(6S)-2-(3-chloro-4-fluorobenzyl)-8-ethyl-10-hydroxy-N,6-dimethyl-1,9-dioxo-1,2,6,7,8,9-hexahydropyrazino[1',2':1,5]pyrrolo[2,3-d]pyridazine-4-carboxamide 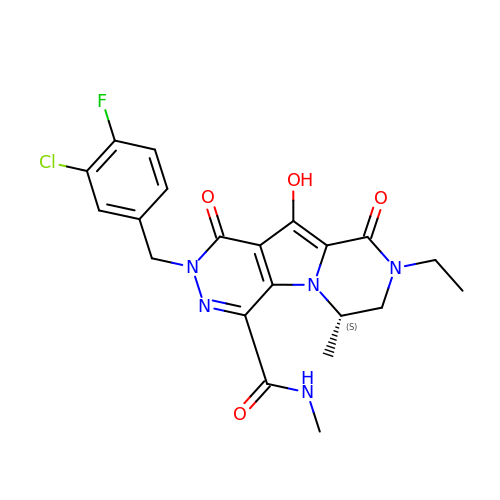| C21 H21 Cl F N5 O4 | JSRREMIKIHJGAA-JTQLQIEISA-N>MTMPYYASAEQIMRDRSELARKGIARGRSVVVLTFRDGVLFVAENPSTALHKVSELYDRLGFAAVGKYNEFENLRRAGIVHADMRGYSYDRRDVTGRSLANAYAQTLGTIFTEQPKPYEVEICVAEVGRVGSPKAPQLYRITYDGSIVDEQHFVVMGGTTEPIATAMRESYRADLDLEAAVGIAVNALRQGGAGEGEKRNVDVASLEVAVLDQSRPRRAFRRIAGTALEQLVPAEPAAASESAPEPKPDTETKPADTQD[7x];>TTIVALTYKGGVLLAGDRRATQGNLIASRDVEKVYVTDEYSAAGIAGTAGIAIELVRLFAVELEHYEKIEGVPLTFDGKANRLASMVRGNLGAAMQGLAVVPLLVGYDLDADDESRAGRIVSYDVVGGRYEERAGYHAVGSGSLFAKSALKKIYSPDSDEETALRAAIESLYDAADDDSATGGPDLTRGIYPTAVTITQAGAVHVSEETTSELARR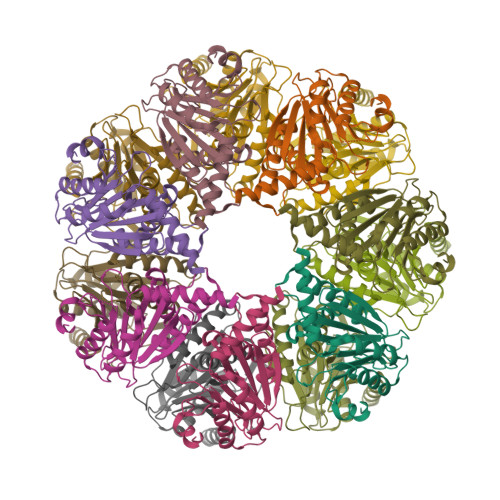IVAERTEQGGSARHHHHHH[7x]> MGAQVSSQKVGAHENSNGAYGGSTINYTTINYYRDSASNAASKQDFSQDPSKFTEPIKDVLIKTAPMLNSPNIEACGYSDRVLQLTLGNSTITAQEAANSVVAYGRWPEYLRDSEANPVDQPTEPEVAACRFYTLDTVSWTKESRGWWWKLPDALRDMGLFGQNMYYHYLGRSGYTVHVQCNASKFHQGALGVFAVPEMCLAGDSNTTTMHTSYQNANPGEKGGTFTGTFTPDNNQTSPARRFCPVDYLLGNGTLLGNAFVFPHQIINLRTNNCATLVLPYVNSLSIDSM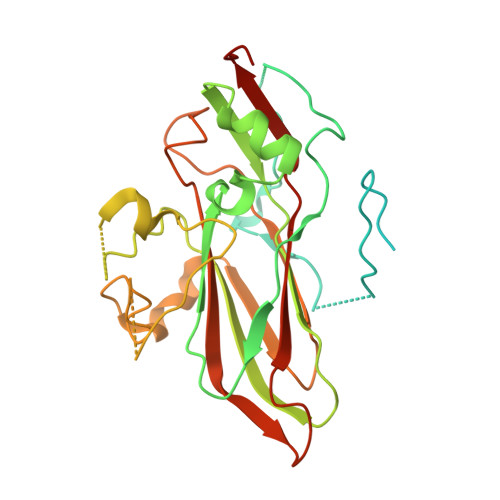VKHNNWGIAILPLAPLNFASESSPEIPITLTIAPMCCEFNGLRNITLPRLQ> NDVGAESKQPLLDIALKGLKRTLPQLEQMDGNSLRENFQEMASGNGPLRSLMTNLQNLNKIPEAKQLNDYVTTLTNIQVGVARFSQWGTCGGEVERWVDKASTHELTQAVKKIHVIAKELKNVTAELEKIEAGAPMPQTMSGPTLGLARFAVSSIPINQQTQVKLSDGMPVPVNTLTFDGKPVALAGSYPKNTPDALEAHMKMLLEKECSCLVVLTSEDQMQAKQLPPYFRGSYTFGEVHTNSQKVSSASQGEAIDQYNMQLSCGEKRYTIPVLHVKNWPDHQPLPSTDQLEYLADRVKNSNQNGAPGRSSSDKHLPMIHCLGGVGRTGTMAAALVLKDNPHSNLEQVRADFRDSRNNRMLEDASQ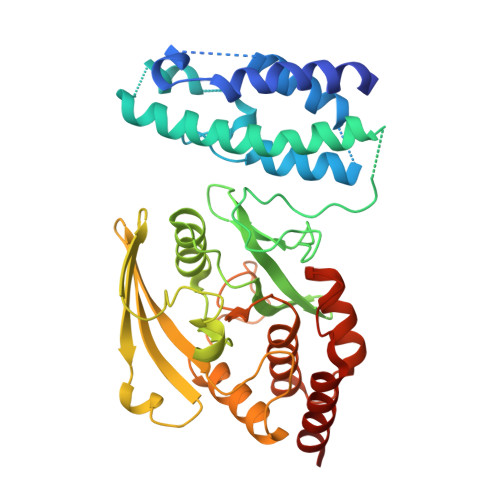FVQLKAMQAQLLMTTAS>GEAGAPCGRISFALRYLYGSDQLVVRILQALDLPAKDSNGFSDPYVKIYLLPDRKKKFQTKVHRKTLNPIFNETFQFSVPLAELAQRKLHFSVYDFDRFSRHDLIGQVVLDNLLELAEQPPDRPLWRDILEGGSEKADLGELNFSLCYLPTAGLLTVTIIKASNLKAMDLTG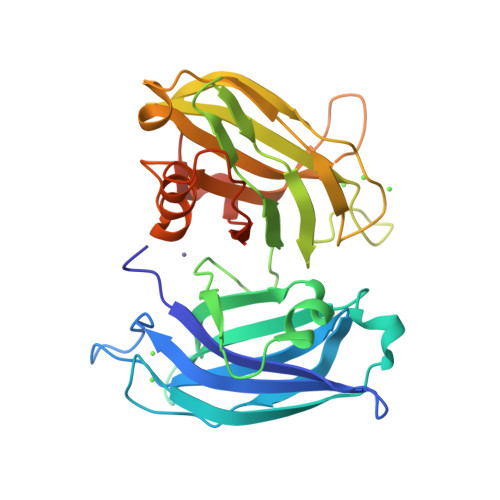FSDPYVKASLISEGRRLKKRKTSIKKNTLNPTYNEALVFDVAPESVENVGLSIAVVDYDCIGHNEVIGVCRVGPEAADPHGREHWAEMLANPRKPVEHWHQLVEEKTLSSFTKGGKGLSEKENS[3x]> MSTAEFAQLLENSILSPDQNIRLTSETQLKKLSNDNFLQFAGLSSQVLIDENTKLEGRILAALTLKNELVSKDSVKTQQFAQRWITQVSPEAKNQIKTNALTALVSIEPRIANAAAQLIAAIADIELPHGAWPELMKIMVDNTGAEQPENVKRASLLALGYMCESADPQSQALVSSSNNILIAIVQGAQSTETSKAVRLAALNALADSLIFIKNNMEREGERNYLMQVVCEATQAEDIEVQAAAFGCLCKIMSLYYTFMKPYMEQALYALTIATMKSPNDKVASMTVEFWSTICEEEIDIAYELAQFPQSPLQSYNFALSSIKDVVPNLLNLLTRQNEDPEDDDWNVSMSAGACLQLFAQNCGNHILEPVLEFVEQNITADNWRNREAAVMAFGSIMDGPDKVQRTYYVHQALPSILNLMNDQSLQVKETTAWCIGRIADSVAESIDPQQHLPGVVQACLIGLQDHPKVATNCSWTIINLVEQLAEATPSPIYNFYPALVDGLIGAANRIDNEFNARASAFSALTTMVEYATDTVAETSASISTFVMDKLGQTMSVDENQLTLEDAQSLQELQSNILTVLAAVIRKSPSSVEPVADMLMGLFFRLLEKKDSAFIEDDVFYAISALAASLGKGFEKYLETFSPYLLKALNQVDSPVSITAVGFIADISNSLEEDFRRYSDAMMNVLAQMISNPNARRELKPAVLSVFGDIASNIGADFIPYLNDIMALCVAAQNTKPENGTLEALDYQIKVLEAVLDAYVGIVAGLHDKPEALFPYVGTIFQFIAQVAEDPQLYSEDATSRAAVGLIGDIAAMFPDGSIKQFYGQDWVIDYIKRTRSGQLFSQATKDTARWAREQQKRQLSL;> MSSNTSSVMSSPRVEKRSFSSTLKSFFTNPNKKRPSSKKVFSSNLSYANHLEESDVEDTLHVNKRKRVSGTSQHSDSLTQNNNNAPIIIYGTENTERPPLLPILPIQRLRLLREKQRVRNMRELGLIQSTEFPSITSSVILGSQSKSDEGGSYLCTSSTPSPIKNGSCTRQLAGKSGEDTNVGLPILKSLKNRSNRKRFHSQSKGTVWSANFEYDLSEYDAIQKKDNKDKEGNAGGDQKTSENRNNIKSSISNGNLATGPNLTSEIEDLRADINSNRLSNPQKNLLLKGPASTVAKTAPIQESFVPNSERSGTPTLKKNIEPKKDKESIVLPTVGFDFIKDNETPSKKTSPKATSSAGAVFKSSVEMGKTDKSTKTAEAPTLSFNFSQKANKTKAVDNTVPSTTLFNFGGKSDTVTSASQPFKFGKTSEKSENHTESDAPPKSTAPIFSFGKQEENGDEGDDENEPKRKRRLPVSEDTNTKPLFDFGKTGDQKETKKGESEKDASGKPSFVFGASDKQAEGTPLFTFGKKADVTSNIDSSAQFTFGKAATAKETHTKPSETPATIVKKPTFTFGQSTSENKISEGSAKPTFSFSKSEEERKSSPISNEAAKPSFSFPGKPVDVQAPTDDKTLKPTFSFTEPAQKDSSVVSEPKKPSFTFASSKTSQPKPLFSFGKSDAAKEPPGSNTSFSFTKPPANETDKRPTPPSFTFGGSTTNNTTTTSTKPSFSFGAPESMKSTASTAAANTEKLSNGFSFTKFNHNKEKSNSPTSFFDGSASSTPIPVLGKPTDATGN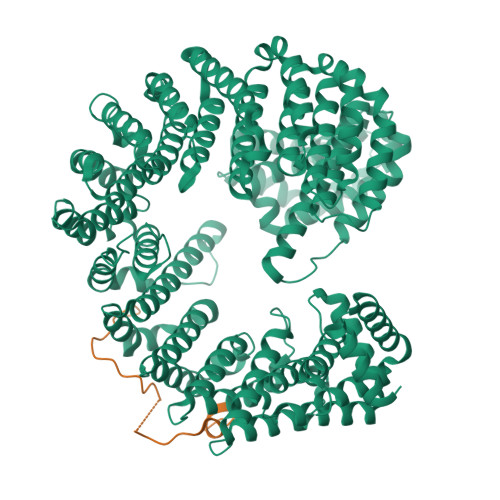TTSKSAFSFGTANTNGTNASANSTSFSFNAPATGNGTTTTSNTSGTNIAGTFNVGKPDQSIASGNTNGAGSAFGFSSSGTAATGAASNQSSFNFGNNGAGGLNPFTSATSSTNANAGLFNKPPSTNAQNVNVPSAFNFTGNNSTPGGGSVFNMNGNTNANTVFAGSNNQPHQSQTPSFNTNSSFTPSTVPNINFSGLNGGITNTATNALRPSDIFGANAASGSNSNVTNPSSIFGGAGGVPTTSFGQPQSAPNQMGMGTNNGMSMGGGVMANRKIARMRHSKR The AAA+ (ATPases Associated with various cellular Activities) family member Rea1 (or Midasin) consists of nearly 5000 amino acids and generates force to mechanically remove assembly factors. Rea1 consists of an N-terminal α-helical domain (NTD), a ring of six AAA+ domains, and the C-terminal tail. The Rea1 tail is subdivided into an α-helical linker region, a D/E-rich region, and a MIDAS (Metal-Ion-Dependent Adhesion Site) domain which is responsible for the interaction with the Ytm1 and Rsa4 substrates. Rea1 pulls out the Ytm1 complex to promote the transfer of pre-60S particles from the nucleolus to the nucleoplasm.

In order to gain insight into nucleotide-dependent Rea1 linker remodelling, we determined the Rea1 cryoEM structure in the presence of the non-hydrolysable ATP analogue AMPPNP to a resolution of 4.3 Å. The Rea1 AMPPNP state is highly similar to the ADP state. The Rea1 ADP structure can be docked into the cryoEM density with minimal adjustments. The fact that there were no significant conformational changes in the AAA+ ring compared to the ADP state reinforces our interpretation of the AAA2L-H2α insert as an auto-inhibitory element that prevents movement between the AAA+ modules of the ring. Since there was no evidence for linker remodelling in the AMPPNP state, we decided to investigate the alternative APO and ATP nucleotide states by negative stain electron microscopy. The Rea1 and Rea1_ΔAAA2L-H2α AMPPNP structures provide strong evidence for the idea that the AAA2L-H2α insert interferes with the nucleotide-dependent conformational changes of the AAA3 and AAA4 modules that create the MIDAS domain binding site.

> XXXXXXXXXXXXXXXXXXXXXXXXXXXXXXXXXXXXXXXXXXXXXXXXXXXXXXXXXXXXXXXXXXXXXXXXXXXXXXXXXXXXXXXXXXXXXXXXXXXXXXXXXXXXXXXXXXXXXXXXXXXXXXXXXXXXXXXXXXXXXXXXXXXXXXXXXXXXXXXXXXXXXXXXXXXXXXXXXXXXXXXXXXXXXXPSVPECFTIEKKSSYFIIEPQDLSTKVASICGVIVPKVHTIHDKVFYPLTFVPTHKTVSSLRQLGRKIQNSTPIMLIGKAGSGKTFLINELSKYMGCHDSIVKIHLGEQTDAKLLIGTYTSGDKPGTFEWRAGVLATAVKEGRWVLIEDIDKAPTDVLSILLSLLEKRELTIPSRGETVKAANGFQLISTVRINEDHQKDSSNKIYNLNMIGMRIWNVIELEEPSEEDLTHILAQKFPILTNLIPKLIDSYKNVKSIYMNTKFISLNKGAHTRVVSVRDLIKLCERLDILFKNNGINKPDQLIQSSVYDSIFSEAADCFAGAIGEFKALEPIIQAIGESLDIASSRISLFLTQHVPTLENLDDSIKIGRAVLLKEKLNIQKKSMNSTLFAFTNHSLRLMEQISVCIQMTEPVLLVGETGTGKTTVVQQLAKMLAKKLTVINVSQQTETGDLLGGYKPVNSKTVAVPIQENFETLFNATFSLKKNEKFHKMLHRCFNKNQWKNVVKLWNEAYKMAQSILKITNTENENENAKKKKRRLNTHEKKLLLDKWADFNDSVKKFEAQSSSIENSFVFNFVEGSLVKTIRAGEWLLLDEVNLATADTLESISDLLTEPDSRSILLSEKGDAEPIKAHPDFRIFACMNPATDVGKRDLPMGIRSRFTEIYVHSPERDITDLLSIIDKYIGKYSVSDEWVGNDIAELYLEAKKLSDNNTIVDGSNQKPHFSIRTLTRTLLYVTDIIHIYGLRRSLYDGFCMSFLTLLDQKSEAILKPVIEKFTLGRLKNVKSIMSQTPPSPGPDYVQFKHYWMKKGPNTIQEQAHYIITPFVEKNMMNLVRATSGKRFPVLIQGPTSSGKTSMIKYLADITGHKFVRINNHEHTDLQEYLGTYVTDDTGKLSFKEGVLVEALRKGYWIVLDELNLAPTDVLEALNRLLDDNRELFIPETQEVVHPHPDFLLFATQNPPGIYGGRKILSRAFRNRFLELHFDDIPQDELEIILRERCQIAPSYAKKIVEVYRQLSIERSASRLFEQKNSFATLRDLFRWALRDAVGYEQLAASGYMLLAERCRTPQEKVTVKKTLEKVMKVKLDMDQYYASLEDKSLEAIGSVTWTKGMRRLSVLVSSCLKNKEPVLLVGETGCGKTTICQLLAQFMGRELITLNAHQNTETGDILGAQRPVRNRSEIQYKLIKSLKTALNIANDQDVDLKELLQLYSKSDNKNIAEDVQLEIQKLRDSLNVLFEWSDGPLIQAMRTGNFFLLDEISLADDSVLERLNSVLEPERSLLLAEQGSSDSLVTASENFQFFATMNPGGDYGKKELSPALRNRFTEIWVPSMEDFNDVNMIVSSRLLEDLKDLANPIVKFSEWFGKKLGGGNATSGVISLRDILAWVEFINKVFPKIQNKSTALIQGASMVFIDALGTNNTAYLAENENDLKSLRTECIIQLLKLCGDDLELQQIETNEIIVTQDELQVGMFKIPRFPDAQSSSFNLTAPTTASNLVRVVRAMQVHKPILLEGSPGVGKTSLITALANITGNKLTRINLSEQTDLVDLFGADAPGERSGEFLWHDAPFLRAMKKGEWVLLDEMNLASQSVLEGLNACLDHRGEAYIPELDISFSCHPNFLVFAAQNPQYQGGGRKGLPKSFVNRFSVVFIDMLTSDDLLLIAKHLYPSIEPDIIAKMIKLMSTLEDQVCKRKLWGNSGSPWEFNLRDTLRWLKLLNQYSICEDVDVFDFVDIIVKQRFRTISDKNKAQLLIEDIFGKFSTKENFFKLTEDYVQINNEVALRNPHYRYPITQNLFPLECNVAVYESVLKAINNNWPLVLVGPSNSGKTETIRFLASILGPRVDVFSMNSDIDSMDILGGYEQVDLTRQISYITEELTNIVREIISMNMKLSPNATAIMEGLNLLKYLLNNIVTPEKFQDFRNRFNRFFSHLEGHPLLKTMSMNIEKMTEIITKEASVKFEWFDGMLVKAVEKGHWLILDNANLCSPSVLDRLNSLLEIDGSLLINECSQEDGQPRVLKPHPNFRLFLTMDPKYGELSRAMRNRGVEIYIDELHSRSTAFDRLTLGFELGENIDFVSIDDGIKKIKLNEPDMSIPLKHYVPSYLSRPCIFAQVHDILLLSDEEPIEESLAAVIPISHLGEVGKWANNVLNCTEYSEKKIAERLYVFITFLTDMGVLEKINNLYKPANLKFQKALGLHDKQLTEETVSLTLNEYVLPTVSKYSDKIKSPESLYLLSSLRLLLNSLNALKLINEKSTHGKIDELTYIELSAAAFNGRHLKNIPRIPIFCILYNILTVMSENLKTESLFCGSNQYQYYWDLLVIVIAALETAVTKDEARLRVYKELIDSWIASVKSKSDIEITPFLNINLEFTDVLQLSRGHSITLLWDIFRKNYPTTSNSWLAFEKLINLSEKFDKVRLLQFSESYNSIKDLMDVFRLLNDDVLNNKLSEFNLLLSKLEDGINELELISNKFLNKRKHYFADEFDNLIRYTFSVDTAELIKELAPASSLATQKLTKLITNKYNYPPIFDVLWTEKNAKLTSFTSTIFSSQFLEDVVRKSNNLKSFSGNQIKQSISDAELLLSSTIKCSPNLLKSQMEYYKNMLLSWLRKVIDIHVGGDCLKLTLKELCSLIEEKTASETRVTFAEYIFPALDLAESSKSLEELGEAWITFGTGLLLLFVPDSPYDPAIHDYVLYDLFLKTKTFSQNLMKSWRNVRKVISGDEEIFTEKLINTISDDDAPQSPRVYRTGMSIDSLFDEWMAFLSSTMSSRQIKELVSSYKCNSDQSDRRLEMLQQNSAHFLNRLESGYSKFADLNDILAGYIYSINFGFDLLKLQKSKDRASFQISPLWSMDPINISCAENVLSAYHELSRFFKKGDMEDTSIEKVLMYFLTLFKFHKRDTNLLEIFEAALYTLYSRWSVRRFRQEQEENEKSNMFKFNDNSDDYEADFRKLFPDYEDTALVTNEKDISSPENLDDIYFKLADTYISVFDKDHDANFSSELKSGAIITTILSEDLKNTRIEELKSGSLSAVINTLDAETQSFKNTEVFGNIDFYHDFSIPEFQKAGDIIETVLKSVLKLLKQWPEHATLKELYRVSQEFLNYPIKTPLARQLQKIEQIYTYLAEWEKYASSEVSLNNTVKLITDLIVSWRKLELRTWKGLFNSEDAKTRKSIGKWWFYLYESIVISNFVSEKKETAPNATLLVSSLNLFFSKSTLGEFNARLDLVKAFYKHIQLIGLRSSKIAGLLHNTIKFYYQFKPLIDERITNGKKSLEKEIDDIILLASWKDVNVDALKQSSRKSHNNLYKIVRKYRDLLNGDAKTIIEAGLLYXXXXXXXXXXXXXXXXXXXXXXXXXXXXXXXXRNIDTVASNMDSYLEKISSQEFPNFADLASDFYAEAERLRKETPNVYTKENKKRLAYLKTQKSKLLGDALKELRRIGLKVNFREDIQKVQSSTTTILANIAPFNNEYLNSSDAFFFKILDLLPKLRSAASNPSDDIPVAAIERGMALAQSLMFSLITVRHPLSEFTNDYCKINGMMLDLEHFTCLKGDIVHSSLKANVDNVRLFEKWLPSLLDYAAQTLSVISKYSATSEQQKILLDAKSTLSSFFVHFNSSRIFDSSFIESYSRFELFINELLKKLENAKETGNAFVFDIIIEWIKANKGGPIKKEQKRGPSVEDVEQAFRRTFTSIILSFQKVIGDGIESISETDDNWLSASFKKVMVNVKLLRSSVVSKNIETALSLLKDFDFTTTESIYVKSVISFTLPVITRYYNAMTVVLERSRIYYTNTSRGMYILSTILHSLAKNGFCSPQPPSEEVDDKNLQEGTGLGDGEGAQNNNKDVEQDEDLTEDAQNENKEQQDKDERDDENEDDAVEMEGDMAGELEDLSNGEENDDEDTDSEEEELDEEIDDLNEDDPNAIDDKMWDDKASDNSKEKDTDQNLDGKNQEEDVQAAENDEQQRDNKEGGDEDPNAPEDGDEEIENDENAEEENDVGEQEDEVKDEEGEDLEANVPEIETLDLPEDMNLDSEHEESDEDVDMSDGMPDDLNKEEVGNEDEEVKQESGIESDNENDEPGPEEDAGETETALDEEEGAEEDVDMTNDEGKEDEENGPEEQAMSDEEELKQDAAMEENKEKGGEQNTEGLDGVEEKADTEDIDQEAAVQQDSGSKGAGADATDTQEQDDVGGSGTTQNTYEEDQEDVTKNNEESREEATAALKQLGDSMKEYHRRRQDIKEAQTNGEEDENLEKNNERPDEFEHVEGANTETDTQALGSATQDQLQTIDEDMAIDDDREEQEVDQKELVEDADDEKMDIDEEEMLSDIDAHDANNDVDSKKSGFIGKRKSEEDFENELSNEHFSADQEDDSEIQSLIENIEDNPPDASASLTPERSLEESRELWHKSEISTADLVSRLGEQLRLILEPTLATKLKGDYKTGKRLNMKRIIPYIASQFRKDKIWLRRTKPSKRQYQIMIALDDSKSMSESKCVKLAFDSLCLVSKTLTQLEAGGLSIVKFGENIKEVHSFDQQFSNESGARAFQWFGFQETKTDVKKLVAESTKIFERARAMVHNDQWQLEIVISDGICEDHETIQKLVRRARENKIMLVFVIIDGITSNESILDMSQVNYIPDQYGNPQLKITKYLDTFPFEFYVVVHDISELPEMLSLILRQYFTDLASS> CTKSI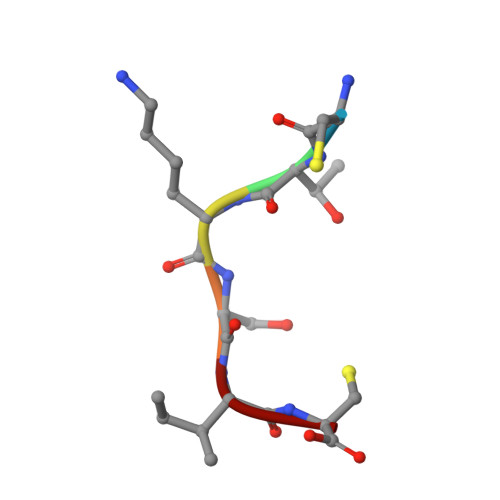C>DALKVNRAPVGVEPQEVHKWLQSFNWDFKENRTKYPTKYHMANETKEQFKVIAKEYARMEAAKDERQFGTLLDGLTRLGAGNKVHPRWGETMKVISNFLEVGEYNAIAASAMLWDSATAAEQKNGYLAQVLDEIRHTHQCAFINHYYSKHYHDPAGHNDARRTRAIGPLWKGMKRVFADGFISGDAVECSVNLQLVGEACFTNPLIVAVTEWASANGDEITPTVFLSVETDELRHMANGYQTVVSIANDPASAKFLNTDLNNAFWTQQKYFTPVLGYL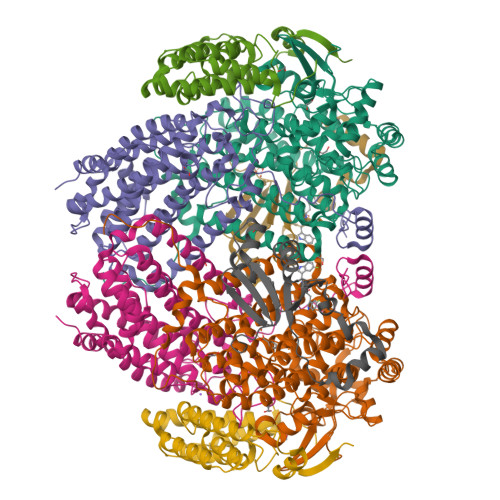FEYGSKFKVEPWVKTWNRWVYEDWGGIWIGRLGKYGVESPASLRDAKRDAYWAHHDLALAAYAMWPLGFARLALPDEEDQAWFEANYPGWADHYGKIFNEWKKLGYEDPKSGFIPYQWLLANGHDVYIDRVSQVPFIPSLAKGTGSLRVHEFNGKKHSLTDDWGERQWLIEPERYECHNVFEQYEGRELSEVIAEGHGVRSDGKTLIAQPHTRGDNLWTLEDIKRAGCVFPDPLAKF[2x];>[2x]PQSSQVTKRGLTDPERAAIIAAAVPDHALDTQRKYHYFIQPRWKRLSEYEQLSCYAQPNPDWIAGGLDWGDWTQKFHGGRPSWGNESTELRTTDWYRHRDPARRWHHPYVKDKSEEARYTQRFLAAYSSEGSIRTIDPYWRDEILNKYFGALLYSEYGLFNAHSSVGRDCLSDTIRQTAVFAALDKVDNAQMIQMERLFIAKLVPGFDASTDVPKKIWTTDPIYSGARATVQEIWQGVQDWNEILWAGHAVYDATFGQFARREFFQRLATVYGDTLTPFFTAQSQTYFQTTRGAIDDLFVYCLANDSEFGAHNRTFLNAWTEHYLASSVAALKDFVGLYAKVEKVAGATDRAGVSEALQRVFGDWKIDYADKIGFRVDVDQKVDAVLAGYKN;>AKREPIHDNSIRTEWEAKIAKLTSVDQATKFIQDFRLAYTSPFRKSYDIDVDYQYIERKIEEKLSVLKTEKLPVADLITKATTGEDAAAVEATWIAKIKAAKSKYEAERIHIEFRQLYKPPVLPVNVFLRTDAALGTVLMEIRNTDYYGTPLEGLRKERGVKVLHLQA[2x];>[2x]SSAHNAYNAGIMQKTGKAFADEFFAEENQVVHESNAVVLVLMKSDEIDAIIEDIVLKGGKAKNPSIVVEDKAGFWWIKADGAIEIDAAEAGELLGKPFSVYDLLINVSSTVGRAYTLGTKFTITSELMGLDRALTDI> GGRALRVLVDMDGVLADFEGGFLRKFRARFPDQPFIALEDRRGFWVSEQYG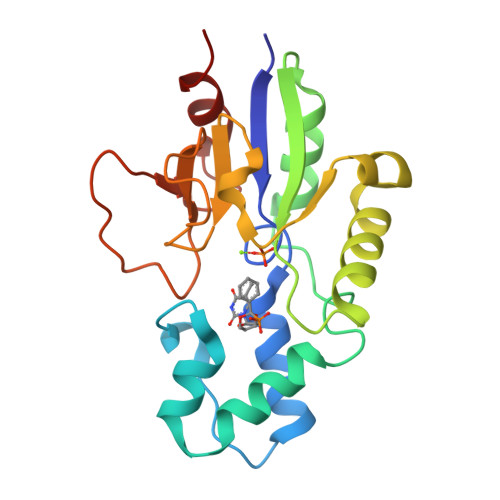RLRPGLSEKAISIWESKNFFFELEPLPGAVEAVKEMASLQNTDVFICTSPIKMFKYCPYEKYAWVEKYFGPDFLEQIVLTRDKTVVSADLLIDDRPDITGAEPTPSWEHVLFTACHNQHLQLQPPRRRLHSWADDWKAILDSKRPC(2~{R},3~{R},4~{S},5~{R},6~{R})-2-[3,5-bis(chloranyl)-4-fluoranyl-phenyl]sulfanyl-6-(hydroxymethyl)-4-[4-(1,3-thiazol-2-yl)-1,2,3-triazol-1-yl]oxane-3,5-diol | C17 H15 Cl2 F N4 O4 S2 | 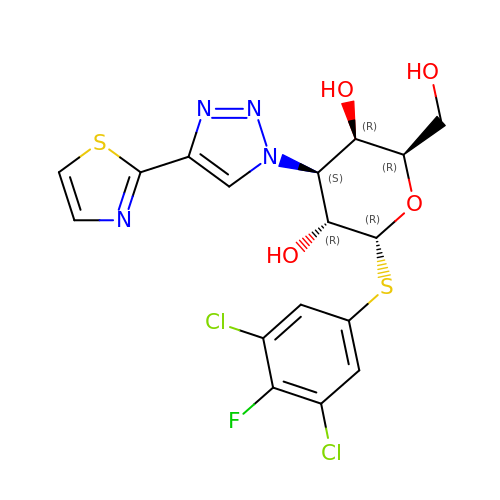QJQNWNOQNZZJCB-YNIRGQLTSA-N>[2x]MYKILEIADVVKVPPEEFGKDLKETVKKILMEKYEGRLDKDVGFVLSIVDVKDIGEGKVVHGDGSAYHPVVFETLVYIPEMYELIEGEVVDVVEFGSFVRLGPLDGLIHVSQIMDDYVSYDPKREAIIGKETGKVLEIGDYVRARIVAISLKAERKRGSKIALTMRQPYLGKLEWIEEEKAKKQNQE;>[2x]MIGKKILGERYVTVSEAAEIMYNRAQIGELSYEQGCALDYLQKFAKLDKEE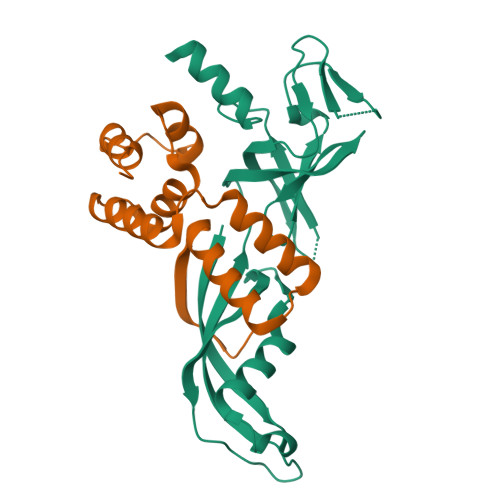AKKLVEELISLGIDEKTAVKIADILPEDLDDLRAIYYKRELPENAEEILEIVRKYI>[4x]MSLEAGAGAPLARYAAWRRAGDFIFLSGIIPVNPLTGTIVNGFQDVPEPVRELLGATGEFSTDAKQGPILAQSWYVLESIRRTVASAGGQMSD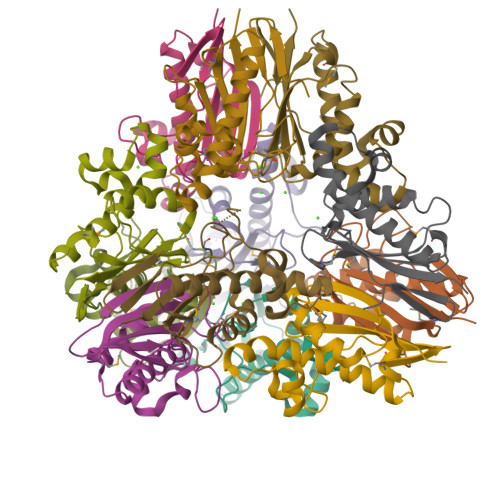VIKLVQYFRNLDHFPYYSRVRKLFYPDQPPVSTVVQVSEMLPDATVLIEVEATVWLPPSFNSEAEGHHHHHH> MPSTSPADKDVPMSILHTHGLSYVNWCMSLAPGLLV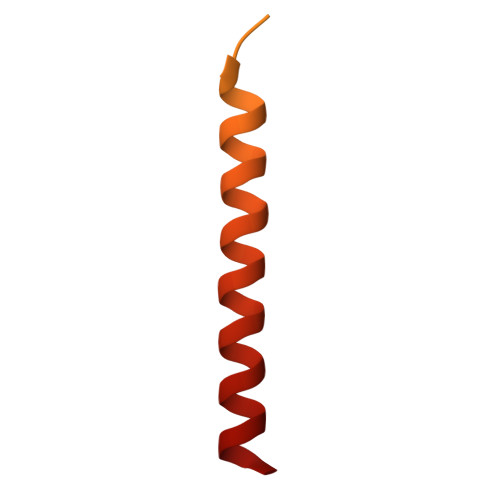FEGFFRARYYRSRVPPSRTVLMNGLKMRMFSLARQQAPKIVHKPVLSPIPEHLRLVKNVAQVQIDMLKLLNAQAAK> CNIKNGRCEQFCKNSADNKVVCSCTEGYRLAENQKSCEPAVPFPCGRVSVSQTSKLTR;> IVGGEDAKPGQFPWQVVLNG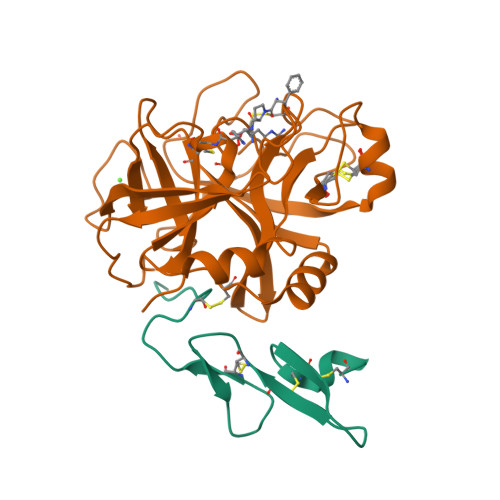KVDAFCGGSIVNEKWIVTAAHCVETGVKITVVAGEHNIEETEHTEQKRNVIRIIPHHNYNAAINTYNHDIALLELDEPLVLNSYVTPICIADKEYTNIFLKFGSGYVSGWGRVFHKGRSALVLQYLRVPLVDRATCLRSTKFTITNNMFCAGFHEGGRDSCQGDSGGPHVTEVEGTSFLTGVISWGEECAMKGKYGIYTKVSRYVNWIKEKTKLT> IFNPDPDDTYIVNMDDFQFTFTMEFEVTVTRGGVHKRTISVDNGRPVVVWDVGDRDPKICKICPDVSSTDIEYVFLDIQKMRLNNLLTQSLWDTQRICVRYACLFLGFDVICDVYHTTDTVRVAYTGQTGKINIQGS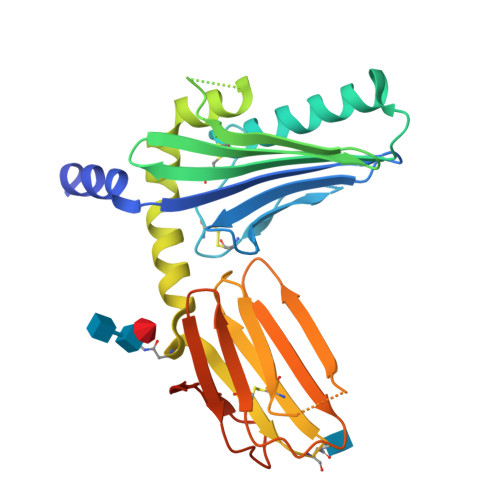GKFSTSDAKEIGTYMIKSNVREIKNRWRSTVQKLKQLAYMNATEVEFWYNTTGLTTCVVTSRSNVPFTVELSLNTNCSAIVTDESTVDCQILTVKAPGSHAQRCYVTSSLGWKGVVTPPSQYRTKRVPVNISSSKWTGIVNWKGNVNR> MKDRFELVSKYQPQGDQPKAIEKLVKGIQEGKKHQTLLGATGTGKTFTVSNLIKEVNKPTLVIAHNKTLAGQLYSEFKEFFPNNAVEYFVSYYDYYQPEAYVPQTDTFIEKDASINDEIDKLRHSATSALFERRDVIIIASVSCIYGLGSPEEYREMVVSLRTEMEIERNELLRKLVDIQYARNDIDFQRGTFRVRGDVVEIFPASRDEHCVRVEFFGDEIERIREVDALTGEILGDRDHVAIFPASHFVTRAEKMEKAIQNIEKELEEQLKVMHENGKLLEAQRLEQRTRYDLEMMREMGFCSGIENYSRHLTLRPPGSTPYTLLDYFPDDFMIVVDESHVTIPQVRGMFNGDQARKQVLVDHGFRLPSALDNRPLRFEEFEKHMHNIVYVSATPGPYEIEHTDEMVEQIIRPTGLLDPLIDVRPIEGQIDDLIGEIQARIERNERVLVTTLTKKMSEDLTDYLKEIGIKVNYLHSEIKTLERIEIIRDLRLGKYDVLVGINLLREGLDIPEVSLVAILDADKEGFLRSERSLIQTIGRAARNAEGRVIMYADKITKSMEIAINETKRRREQQERFNEEHGITPKTINKEIRDVIRATVAAEDKAEYKTKAAPKLSKMTKKERQKVVEQMEHE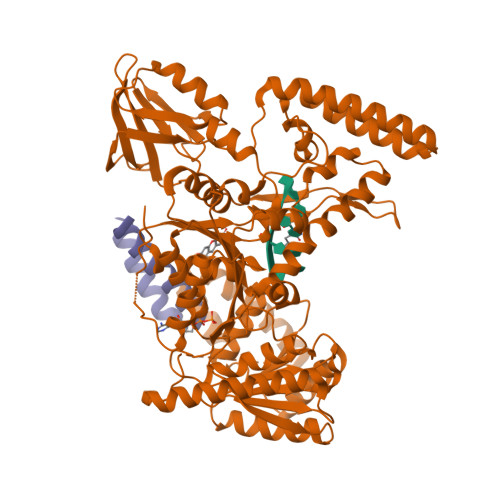MKEAAKALDFERAAELRDLLLELKAEG;> KERQKVVEQMEHEMKEAAKALDFERAAELRDLLLELKA> MRLRISEAVVLFLLGAVAALIGDHSHVVTGTTVYHTDAVPFVWSSPFWFPILVGAATASLAELRLHLPAPRDGVTARQALGGVAAVVGTYVTTALVHAFPVVPVTALVCAAAAITWCVLGDGPGAACGVVIAVIGPAVEIALVQLGVFAYHP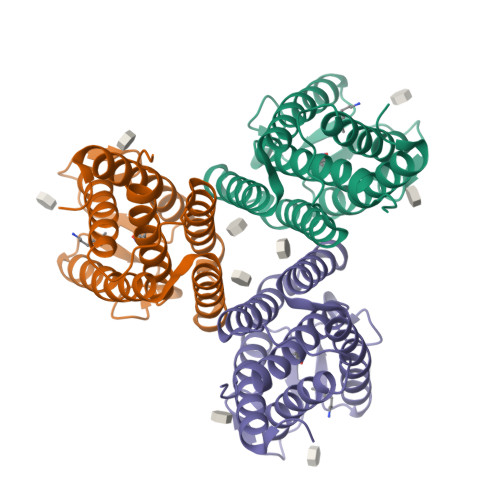DSDGLFGVAPFLAPLYFAFGVVAALLGELAVARRPQLGPPVCDTVSRGPGAGHHHHHH>MSKVKVMTVFGVRPEAIKMAPLILELQKHPEHIESIVCVTAQHRQMLDQVLDVFNIKPDYDLDIMQARQTLNDISVRVLQGLEPVLQEAKPDIVLVHGDTLTTFLASYAAFMQQIKVGHVEAGLRTWNKLSPFPEEMNRQLTGVLADLHFAPTDWSASNLRKENKQDASIFVTGNTVTDVFQYTVRSDYKHEVLDWAQGKRLVLMTAHRRESQGEPHRNIFRAVRRIADEFEDIAIVYPVHPSPAVREPAHEMLGDHPRIKLIDPLDVVDLHNFYPHTHLILTDSGGLQEEAPSFGIPVLVLRETTERPEGIDAGTLELVGTDEEKVYARAKALLSDETTYARMSKAA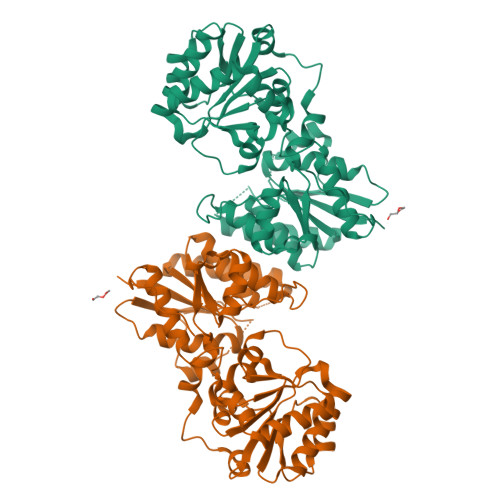NPYGDGKASQRIVSAILHSFGVLEERPEPFHTKFTNLEHHHHHH[2x]Thioredoxins (TRXs) are small oxidoreductases of 10–16 kDa exhibiting a characteristic three dimensional structure classified as TRX fold, composed of a single canonical globular domain comprising a mixed β-sheet surrounded by four α-helices. The redox activity of TRXs is guaranteed by the presence of a solvent-exposed motif (most commonly Trp-Cys-Gly-Pro-Cys) containing two cysteine (Cys) residues that catalyze protein disulfide reduction. Phylogenetic and sequence analyses led to the classification of plant TRXs in different types: TRXs f, m, x, y, and z are chloroplastic, while o-type and h-type are found in mitochondria and cytosol. Here, we describe the novel crystal structure of chloroplastic TRX f2 (CrTRXf2), and a crystal structure of TRX h1 (CrTRXh1) from Chlamydomonas reinhardtii.

The crystal structure of CrTRXf2 was solved at 2.01 Å resolution. The overall structure is a flattened spheroid of 49 Å equatorial diameter and 25 Å polar diameter, and conforms to the classical TRX fold. In CrTRXf2, the first active site Cys (hereafter referred to as CysN) is located at position 38 at the N-terminal kinked tip of α-helix 2. The second catalytic Cys (hereafter referred to as CysC) is located at position 41, and it belongs to the same α-helix 2. In the CrTRXf2 structure, the catalytic Cys are covalently disulfide-bonded in accordance with the non-reducing conditions of the purification and crystallization procedures. Trp37, Gly39, Pro40, and Lys42 of the conserved 37WCGPCK42 motif arch over the disulfide bond, leaving two gates to interact with the solvent. The third cysteine of CrTRXf2, located at position 65, is perfectly conserved amongst f-type TRXs and was shown to be modified by S-glutathionylation. In our structure, Cys65 is likely in the thiol form, since its side chain points inward to a hydrophobic pocket formed by Phe33, Val63 and Ile78. Detailed comparative analysis of the crystal structures of CrTRXf2 with other TRXs revealed that the f-type specifically (i) forms a rougher surface with larger cavities, (ii) orients a crown of electropositive patches on the two opposite sides of the active site disulfide, and (iii) adopts a local flexible hinge downstream of α helix 1. These specific structural features of CrTRXf2 should guide the recognition of specific targets by facilitating target space accommodation, flexibility, and electrostatic interactions.

>MHHHHHHTMGGSVDGQGLLQLDKDTFWPYLEQQQDTLVVVDFYTDWCGPCKLIYPELVKLSQERTDVRFVKVNCNKSNKELGMQLAIKVAPTFHLYRNKTKVADMTGAKMDKLIALINQHQPPKN[3x]1-[4-[[2-(1H-indazol-4-yl)-4-morpholin-4-yl-thieno[3,2-d]pyrimidin-6-yl]methyl]piperazin-1-yl]-6-methyl-hept-5-ene-1,4-dione 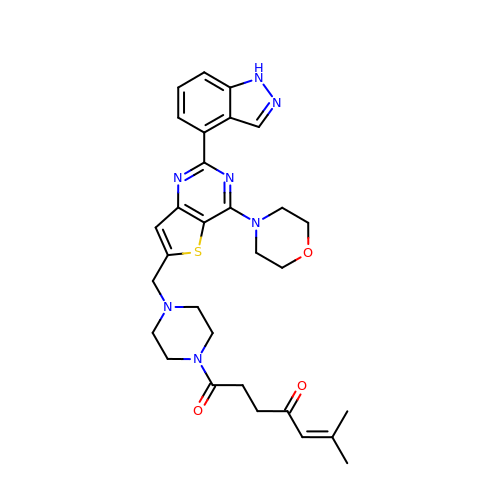| C30 H35 N7 O3 S | DLNUPKDFXMWRFP-UHFFFAOYSA-N> MKKLEITIRPENLEEVKQILSDRGVSGMTIL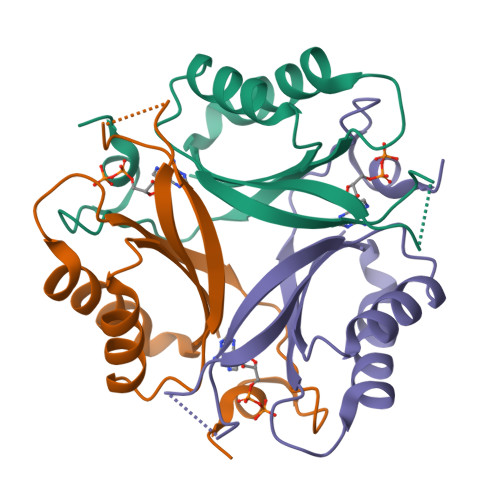SAMGAGNQKGEKTTTILKGGEFHINLLPKIHVITYVKDHLVGNILIDIHERLSTGEVGDGKVIVSPLEEVMRIRTGERGENALSAWSHPQFEK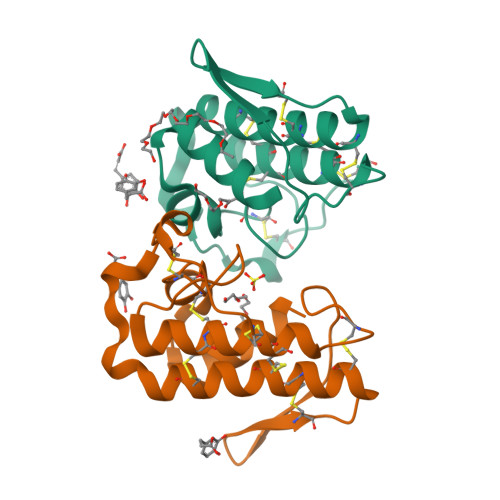>[2x]SLFELGKMILQETGKNPAKSYGAYGCNCGVLGRGKPKDATDRCCYVHKCCYKKLTGCNPKKDRYSYSWKDKTIVCGENNPCLKELCECDKAVAICLRENLGTYNKLYRYHLKPFCKKADDC> EQCSPQQRTTRISGRDGLCVDVYGALTADGSRVILYPCGQQQNQQWTFYPDNTIRSLGKCLATSALSSGSNVVITNCDYLRY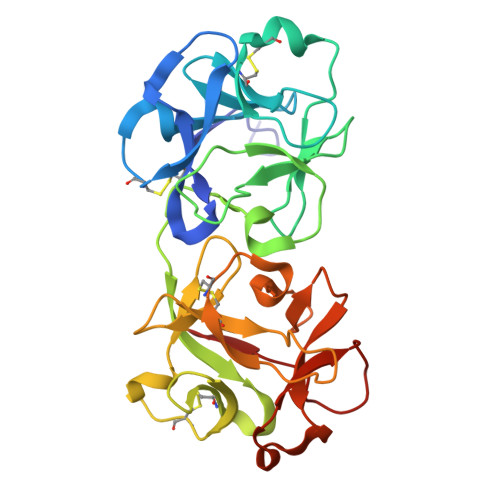DDGWMVSSSGTMMNKSSHLVLTANAATSRTNLTGENNVFAAKQAWRIGNYVEPIVTTIIGLRHMCLEATDNDTNVWLESCVKNKTKQYWALYSDDTIRVNNNRNLCVSSSTDSSSKLIVIRRCDGSINQRWVFTPQGTISNPGYEAVMDVAQNDVYLKKIVLSSATDKGNGQQWTVFY>[2x]GSKKPHPRYQQPPV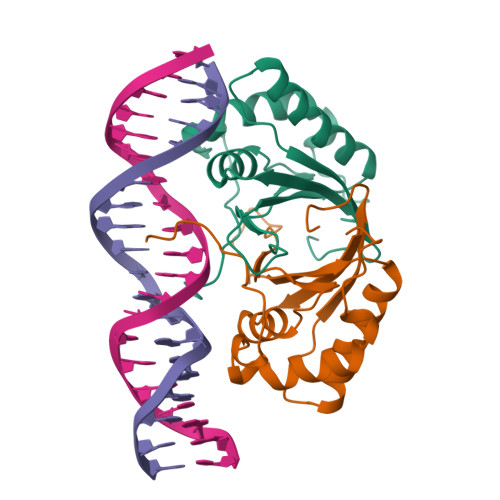PYRQIDDCPAKARPQHIFYQQFLGKDGRRDPKCQWEFAVIFWGNDPYGLKKLSQAFQFGGVKAGPVSCLPHPGPDQSPITYCVYVYCQNAATSKKVQMARLEWEASHPLAGNLQSSIVSFDDPLPLT>[2x]XEVEALEKKVEALEVKVQK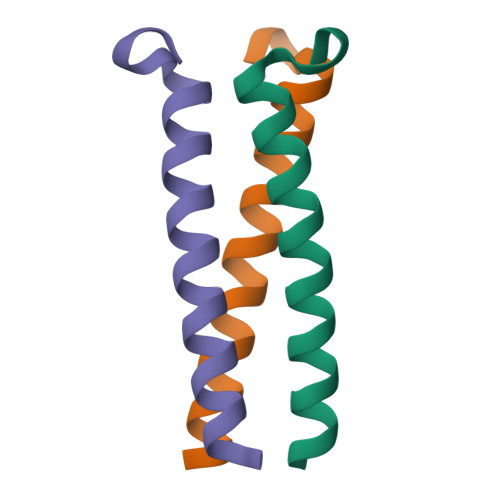LEKKVEALEHGWDGR> MDRSAVDTIRGYCYQVDKTIIEIFSLPQMDDSIDIECIEDVDVYNDGHLTAIQCKYYESTDYNHSVISKPIRLMLSHFKDNKEKGANYYLYGHYKSGQEKLTLPLKVDFFKSNFLTYTEKKIKHEYHIENGLTEEDLQAFLDRLVININAKSFDDQKKETIQIIKNHFQCEDYEAEHYLYSNAFRKTYDISCNKKDRRIKKSDFVESINKSKVLFNIWFYQYEGRKEYLRKLKESFIRRSVNTSPYARFFILEFQDKTDIKTVKDCIYKIQSNWSNLSKRTDRPYSPFLLFHGTSDANLYELKNQLFNEDLIFTDGYPFKGSVFTPKMLIEGFSNKEIHFQFINDI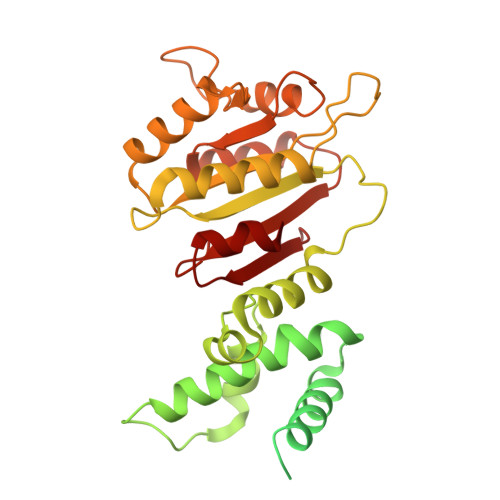DDFNETLNSINIRKEVYQFYTENCLDIPSQLPQVNIQVKDFADIKEIV>[2x]MKTEQQIADIVNRTITPLMQEQAIPGMAVAVIYQGKPYYFTWGKADIANNHPVTQQTLFELGSVSKTFNGVLGGDAIARGEIKLSDPVTKYWPELTGKQWQGIRLLHL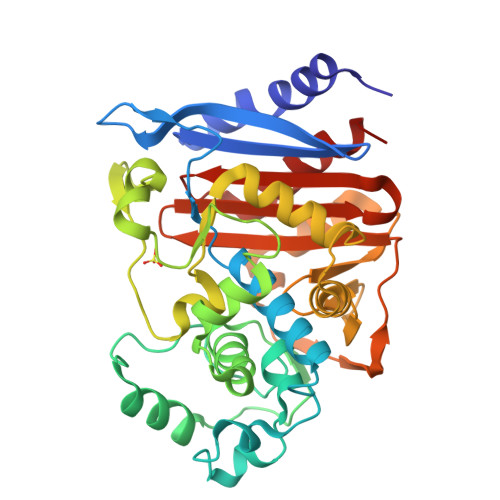ATYTEGGLPLKIPDDVRDKAALLHFYQNWQPQWTPGAKRLYANSSIGLFGALAVKPSGMSYEEAMTRRVLQPLKLAHTWITVPQNEQKDYAWGYREGKPVHSSPGQLDAEAYGVKSSVIDMARWVQANMDASHVQEKTLQQGIALAQSRYWRIGDMYQGLGWEMLNWPLKADSIINGSDSKVALAALPAVEVNPPAPAVKASWVHKTGSTGGFGSYVAFVPEKNLGIVMLANKSYPYPVRVEAAWRILEKLQ> SPNSQYLKTRILDIYTPEQRAGIEKSEDWRQFSRRMDTHFPKLMNELDSVYGNNEALLPMLEMLLAQAWQSYSQRNSSLKDIDIARENNPDWILSNKQVGGVCYVDLFAGDLKGLKDKIPYFQELGLTYLHLMPLFKCPEGKSDGGYAVSSYRDVNPALGTIGDLREVIAALHEAGISAVVDFIFNHTSNEHEWAQRCAAGDPLFDNFYYIFPDRRMPDQYDRTLREI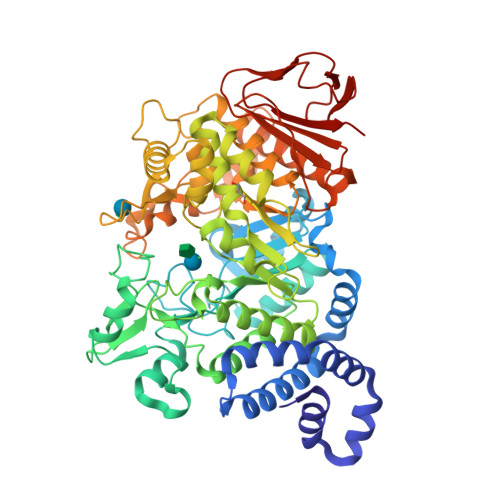FPDQHPGGFSQLEDGRWVWTTFNSFQWDLNYSNPWVFRAMAGEMLFLANLGVDILRMDAVAKIWKQMGTSCENLPQAHALIRAFNAVMRIAAPAVFFKSQAIVHPDQVVQYIGQDECQIGYNPLQMALLWNTLATREVNLLHQALTYRHNLPEHTAWVNYVRSHDDIGWTFADEDAAYLGISGYDHRQFLNRFFVNRFDGSFARGVPFQYNPSTGDCRVSGTAAALVGLAQDDPHAVDRIKLLYSIALSTGGLPLIYLGDEVGTLNDDDWSQDSNKSDDSRWAHRPRYNEALYAQRNDPSTAAGQIYQDLRHMIAVRQSNPRFDGGRLVTFNTNNKHIIGYIRNNALLAFGNFSEYPQTVTAHTLQAMPFKAHDLIGGKTVSLNQDLTLQPYQVMWLEIA> THRLITLADHI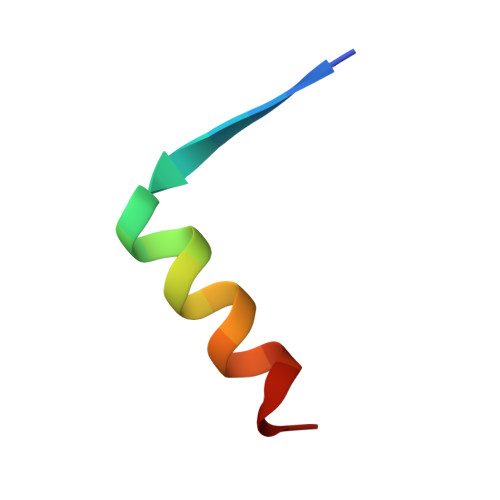AQIITQDFA> HWKTRAVPGAGTFGSAVAGQELPLCGVRAYYPPNAYIPAQVRDWLEFAHRPGLMATVPWTMADEPAERLGIFPVSPSAIAGTGAPISYVISLF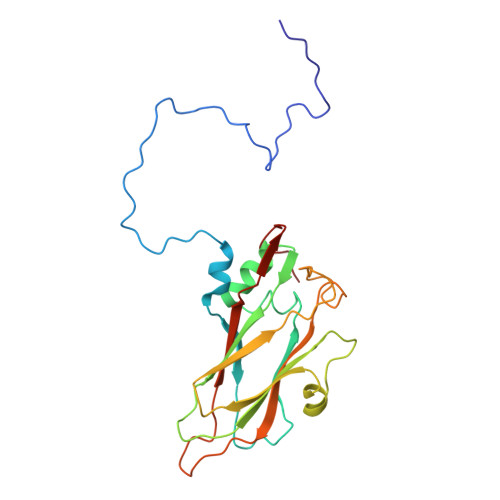SQWRGELAAHLLFTGSAQHYGRLVVCYTPAAPQPPSTMQEAMRGTYTVWDVNAASTLEFTIPFISNSYWKTVDVNNPDALLSTTGYVSIWVQNPLVGPHTAPASALVQAFISAGESFNVRLMQNPALTSQ>[4x]MSLTPRNATVAVIGAGDYIGAEIAKKFAAEGFTVFAGRRNGEKLAPLVAEIEAAGGRIVARSLDARNEDEVTAFLNAADAHAPLEVTIFNVGANVNFPILETTDRVFRKVWEMACWAGFVSGRESARLMLAHGQGKIFFTGATASLRGGSGFAAFASAKFGLRAVAQSM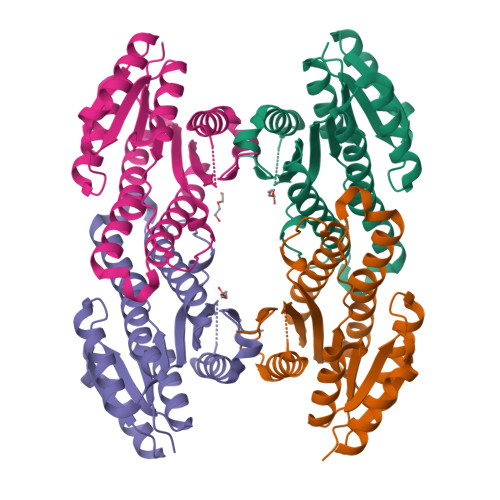ARELMPKNIHVAHLIIDSGVDTAWVRERREQMFGKDALANPDLLMPPAAVAGAYWQLYQQPKSAWTFEMEIRPYGEGHHHHHH>MSTNKVNKERTFLAVKPDGVARGLVGEIIARYEKKGFVLVGLKQLVPTKDLAESHYAEHKERPFFGGLVSFITSGPVVAMVFEGKGVVASARLMIGVTNPLASAPGSIRGDFGVDVGRNIIHGSDSVESANREIALWFKPEELLTEVKPNPNL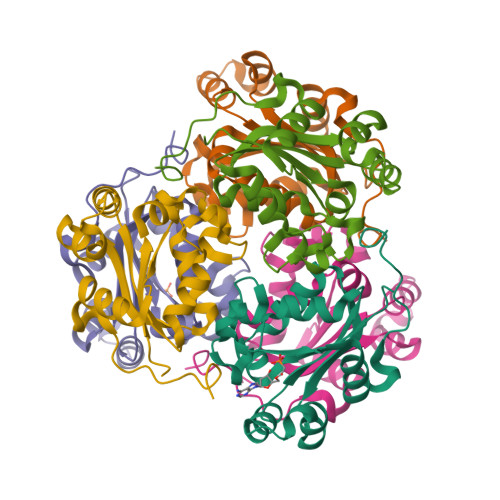YE[6x]> MVKLAFPRELRLLTPSQFTFVFQQPQRAGTPQITILGRLNSLGHPRIGLTVAKKNVRRAHERNRI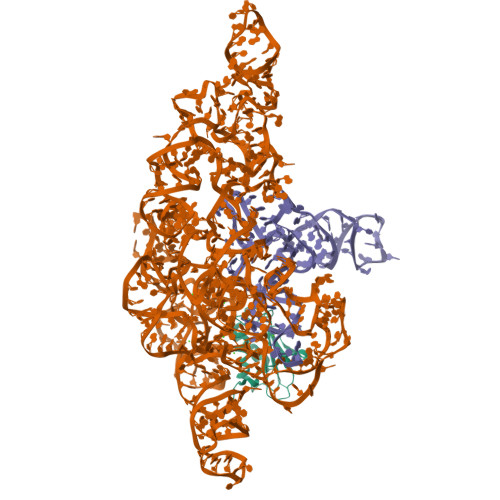KRLTRESFRLRQHELPAMDFVVVAKKGVADLDNRALSEALEKLWRRHCRLARGS3-amino-7-{(3R)-3-[(1S)-1-aminoethyl]pyrrolidin-1-yl}-1-cyclopropyl-6-fluoro-8-methylquinazoline-2,4(1H,3H)-dione 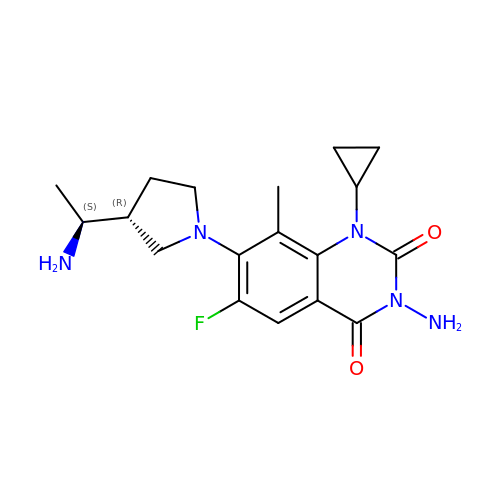| C18 H24 F N5 O2 | SMONLCFJGCJROJ-WDEREUQCSA-N>[4x]STTGIIMENVTAFWEEGFGELLEKVQQSNGDRKHSSDENNVSFSHLCLVGNPVLKNINLNIEKGEMLAITGSTGSGKTSLLMLILGELEASEGIIKHSGRVSFCSQFSWIMPGTIKENIISGVSYDEYRYKSVVKACQLQQDITKFAEQDNTVLGEGGVTLSGGQRARISLARAVYKDADLYLLDSPFGYLDVFTEEQVFESCVCKLMANKTRILVTSKMEHLRKADKILILHQGSS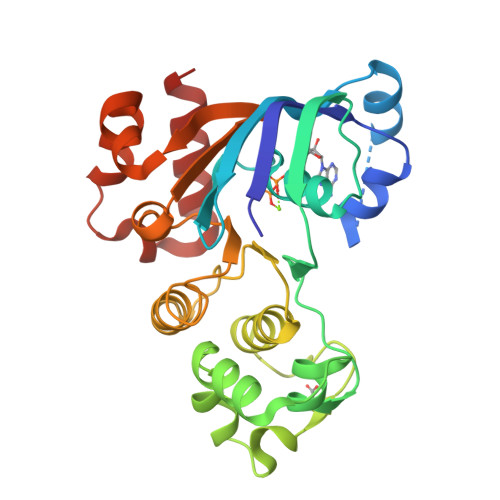YFYGTFSELQSLRPDFSSKLMGYDTFDQFTEERRSSILTETLRRFS> MKQQIILWIGVLLLLIGGVGCKKDQSSCCDKEIIKDVSELTGIISYNTEVKRWYI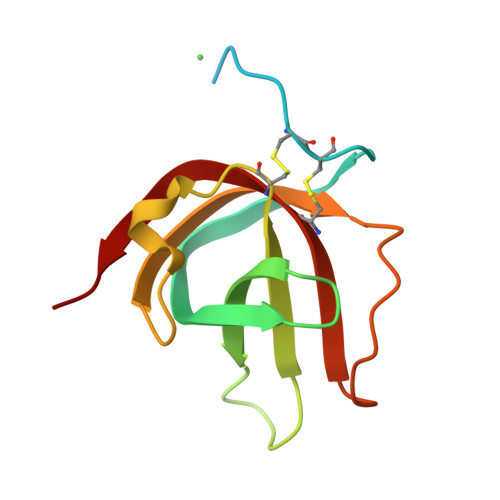SVSDANSYDNVTLYFPCNLDSKYMKEKEKVIFSGQISKSTLKITLPAGTTSYCINLMSINKIN> MRGSHHHHHHGSPPAAPITLWTGPGPSINGFINDTPVIRCFICLTRDSNLVTVNASFVGEGGYRIVSPTQSQFSLIMEFDQFGQLMSTGNINSTTTWGEKPWGNNTVQPRPSHTWKLCMPN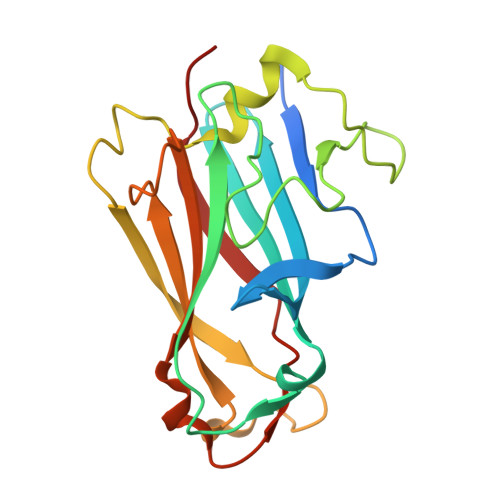REVYSTPAATISRCGLDSIAVDGAPSRSIDCMLIINKPKGVATYTLTFRFLNFNRLSGGTLFKTDVLTFTYVGENQ> GPL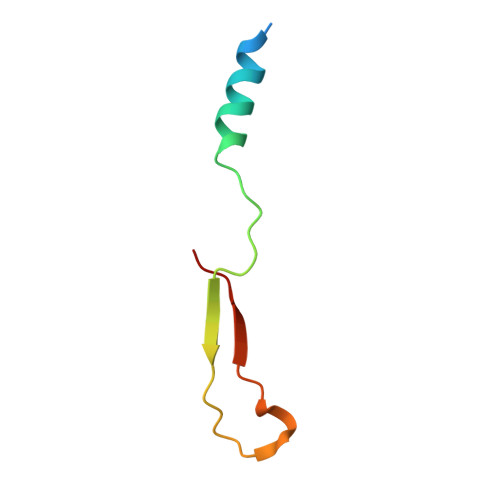GSMQVDSVQRWMEDLKLMTECECMCVLQAKPISLEEDAQGDLILAGGPG>PHIDIKCFPRELDEQQKAALAADITDVIIRHLNSKDSSISIALQQIQPESWQAIWDAEIAPQMEALIKKP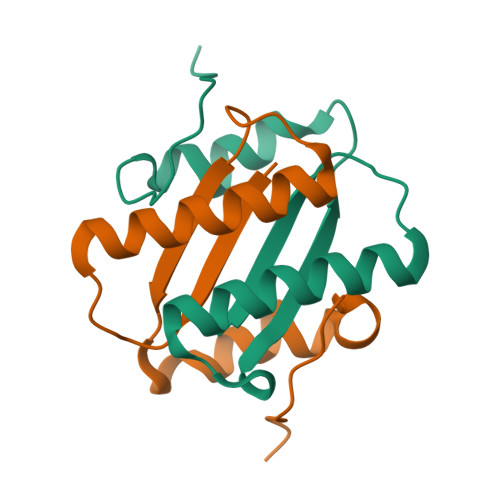GYSMNA[2x]[(2-amino-9-methyl-6-oxo-6,9-dihydro-1H-purin-8-yl)sulfanyl]acetic acid | C8 H9 N5 O3 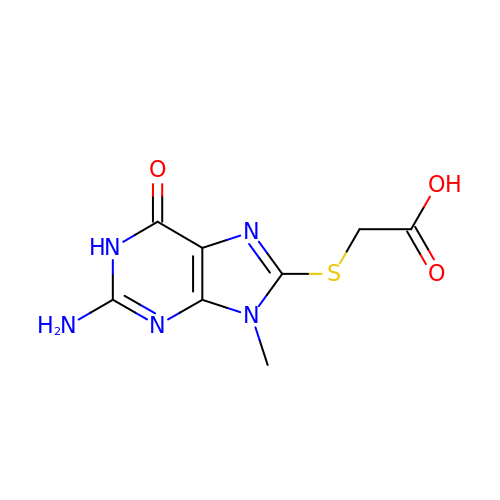S | QISKTUNYOVVFHP-UHFFFAOYSA-N> MACEGAPEVRIGRKPVMNYVLAILTTLMEQGTNQVVVKARGRNINRAVDAVEIVRKRFAKNIEIKDIKIDSQEIEVQTPEGQTRTRRVSSIE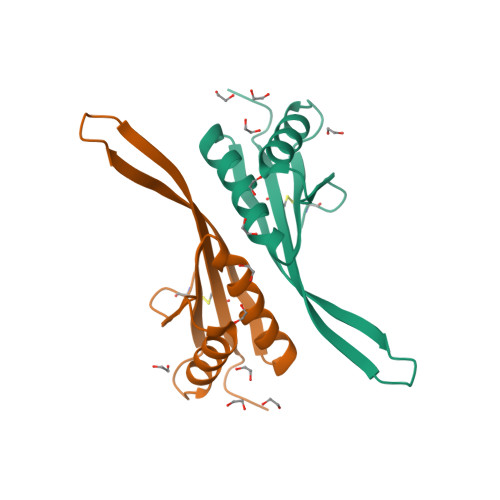ICLEKAGESA7-amino-1-methyl-3-{[(1H-tetrazol-5-yl)amino]methyl}pyrimido[4,5-c]pyridazine-4,5(1H,6H)-dione | 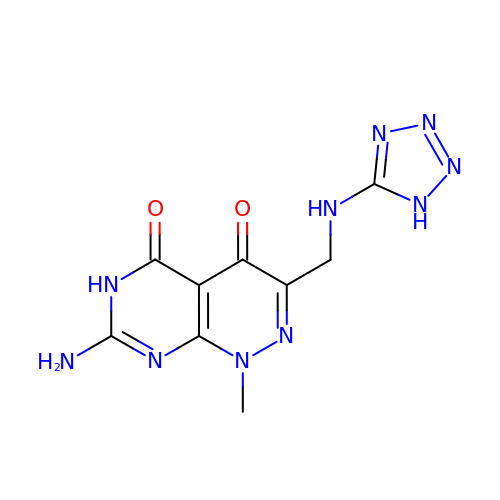C9 H10 N10 O2 | HPEOIAAOXXIKAO-UHFFFAOYSA-N>[2x]QIQKAEQNDVKLAPPTDVRSGYIRLVKNVNYYIDSESIWVDNQEPQIVHFDAVVNLDKGLYVYPEPKRYARSVRQYKILNCANYHLTQVRTDFYDEFWGQGLRAAPKKQKKHTLSLTPDTTLYNAAQIICANYGEAFSVD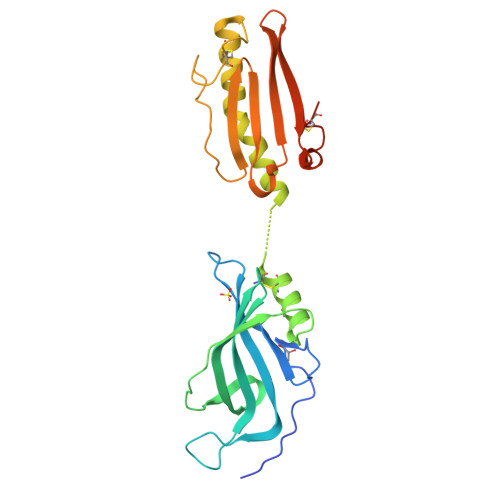KKGGTKKAAVSELLQASAPYKADVELCVYSTNETTNCTGGKNGIAADITTAKGYVKSVTTSNGAITVKGDGTLANMEYILQATGNAATGVTWTTTCKGTDASLFPANFCGSVTQGGHHHHHH>GSHMDYILGRYVKIARYGSGGLVGGGGKEQYVENLVLWENIIKTAYCFITPSSYTAALETANIPEKDFSNCFRFLKENFFIIPGEYNNSTENNRYSRNFLHYQSYGANPVLVQDKLKNAKVVILGCGGIGNHVSVILATSGIGEIILIDNDQIENTNLTRQVLFSEDDVGKNKTEVIKRELLKRNSEISVSEIALNINDYTDLHKVPEADIWVVSADHPFNLINWVNKYCVRANQPYINAGYVNDIAVFGPLYVPGKTGCYECQKVVADLYGSEKENIDHKIKLINSRFKPATFAPV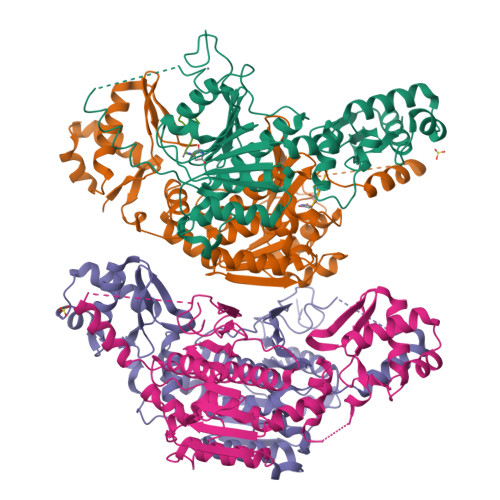NNVAAALCAADVIKFIGKYSEPLSLNKRIGIWSDEIKIHSQNMGRSPVCSVCGNRM[4x];>MRTGNAN[4x]>[6x]MGESERSEAFGIPRDSPLSSGDAAELEQLRREAAVLREQLENAVGSHAPTRSARDIHQLEARIDSLAARNSKLMETLKEARQQLLALREEVDRLGQPPSGYGVLLATHDDDTVDVFTSGRKMRLTCSPNIDAASLKKGQTVRLNEALTVVEAGTFEAVGEISTLREILADGHRALVVGHADEERVVWLADPLIAEDLPDGLPEALNDDTRPRKLRPGDSLLVDTKAGYAFERIPKAEVEDLVLEEVPDVSYADIGGLSRQIEQIRDAVELPFLHKELYREYSLRPPKGVLLYGPPGCGKTLIAKAVANSLAK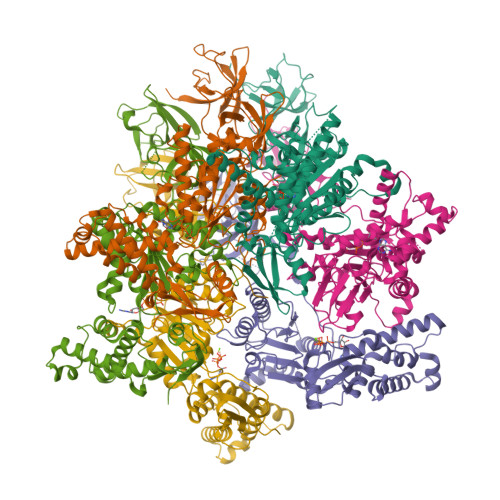KMAEVRGDDAHEAKSYFLNIKGPELLNKFVGETERHIRLIFQRAREKASEGTPVIVFFDEMDSIFRTRGTGVSSDVETTVVPQLLSEIDGVEGLENVIVIGASNREDMIDPAILRPGRLDVKIKIERPDAEAAQDIYSKYLTEFLPVHADDLAEFDGDRSACIKAMIEKVVDRMYAEIDDNRFLEVTYANGDKEVMYFKDFNSGAMIQNVVDRAKKNAIKSVLETGQPGLRIQHLLDSIVDEFAENEDLPNTTNPDDWARISGKKGERIVYIRTLVTGKSSSASRAIDTESNLGQYL;> GSMAQEQTKRGGGGGDDDDIAGSTAAGQERREKLTEETDDLLDEIDDVLEENAEDFVRAYVQKGGQ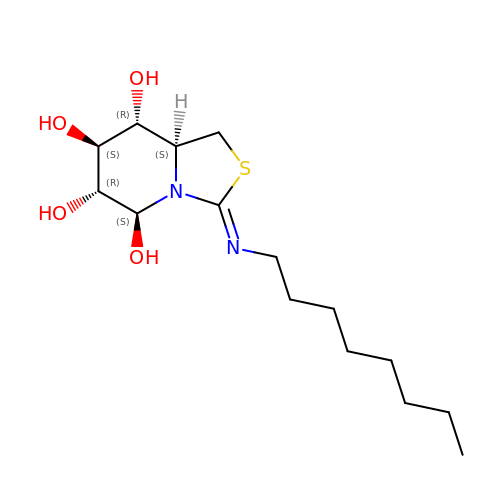(3Z,5S,6R,7S,8R,8aS)-3-(octylimino)hexahydro[1,3]thiazolo[3,4-a]pyridine-5,6,7,8-tetrol | C15 H28 N2 O4 S | HXWFEIXEWVGTGU-KRIYVDMXSA-N>GMGFEEEEVRFRLDDTDKQEISKTLTSVYRSLEEKGYNPI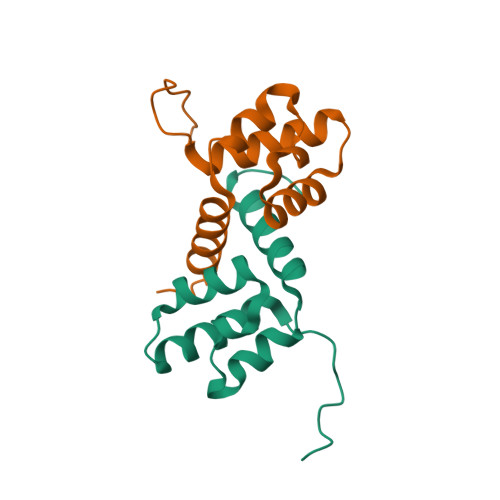NQIIGYVLSGDPAYIPRYNDARNQIRKHERDEIIEELVRYYLKGNGIDL[2x]2-{3'-[AMINO(IMINO)METHYL]BIPHENYL-4-YL}-1H-BENZIMIDAZOLE-5-CARBOXIMIDAMIDE 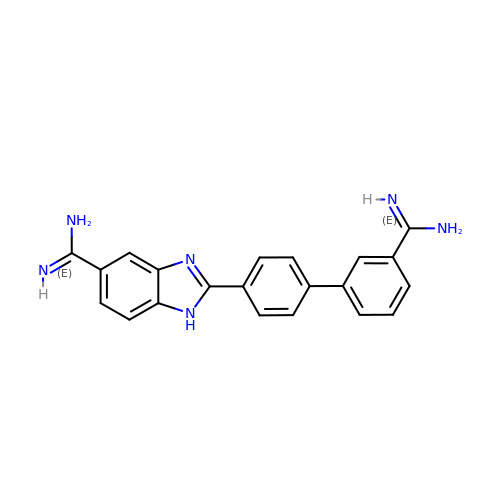| C21 H18 N6 | JTEAXLWMBHFLPI-UHFFFAOYSA-N[(2R)-2-[(E)-octadec-9-enoyl]oxy-3-[oxidanyl-[(1R,2R,3S,4R,5R,6S)-2,3,6-tris(oxidanyl)-4,5-diphosphonooxy-cyclohexyl]oxy-phosphoryl]oxy-propyl] 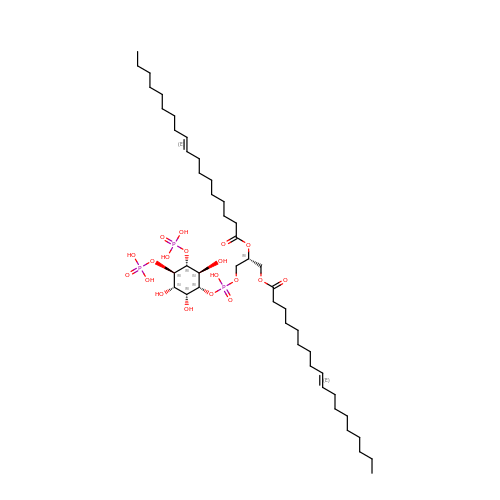(E)-octadec-9-enoate | C45 H85 O19 P3 | IGQSAMXNWMLOOS-ZLFOHRMWSA-N>MAEKNYVMAIDQGTTSSRAIIFDRNGKKIGSSQKEFPQYFPKSGWVEHNANEIWNSVQSVIAGAFIESGIRPEAIAGIGITNQRETTVVWDKTTGQPIANAIVWQSRQSSPIADQLKVDGHTEMIHEKTGLVIDAYFSATKVRWLLDNIEGAQEKADNGELLFGTIDSWLVWKLTDGQVHVTDYSNASRTMLYNIHKLEWDQEILDLLNIPSSMLPEVKSNSEVYGHTRSYEFYGSEVPIAGMAGDQQAALFGQMAFEKGMIKNTYGTGAFIVMNTGEEPQLSDNDLLTTIGYGINGKVYYALEGSIFVAG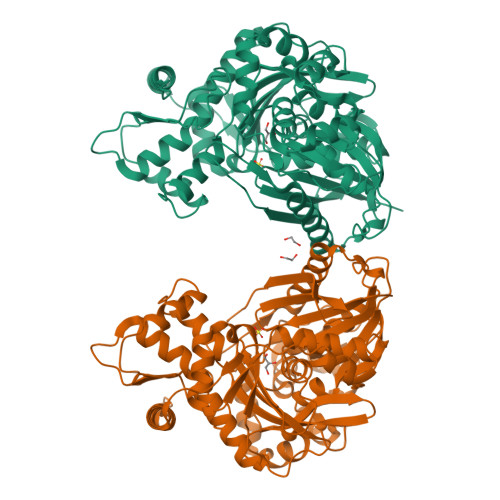SAIQWLRDGLRMIETSPQSEELAAKAKGDNEVYVVPAFTGLGAPYWDSEARGAVFGLTRGTTKEDFVRATLQAVAYQSKDVIDTMKKDSGIDIPLLKVDGGAAKNDLLMQFQADILDIDVQRAANLETTALGAAYLAGLAVGFWKDLDELKSMAEEGQMFTPEMPAEERDNLYEGWKQAVAATQTFKFKAKKEGE[2x]> MAGNDSNLIWLDL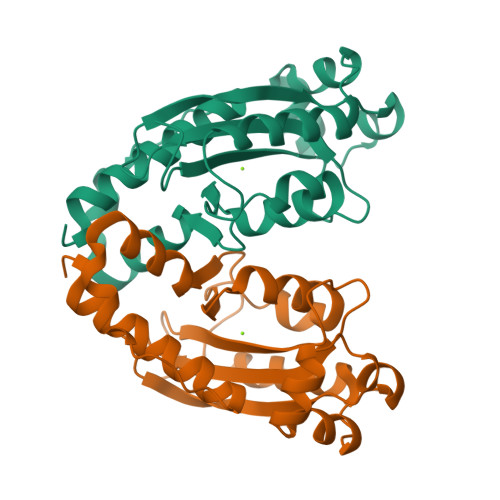EMTGLEPVEDVILEIAIIITDSELNILAQGPIFAISQTDDVLDNMNPWCIEHHGKSGLTQRCRDSEVSLAHATKESLAFVQEWVPQGKSPMCGNSIGQDRRFINKYMPDFEDHFHYRNLDVSTIKELAKRWKPEVLESVVKTGAHLALDDIKESIAELKVYRELFFKL> MNHLGKTEVFLNRFALRPLNPEELRPWRLEVVLDPPPGREEVYPLLAQVARRAGGVTVRMGDGLASWSPPEVLVLEGTLARMGQTYAYRLYPKGRRPLDPKDPGERSVLSALARRLLQERLRRLEGVWVEGLAVYRREHARGPGWRVLGGAVLDLWVSDSGAFLLEVDPAYRILCEMSLEAWLAQGHPLPKRVRNAYDRRTWELLRLGEEDPKELPLPGGLSLLDYH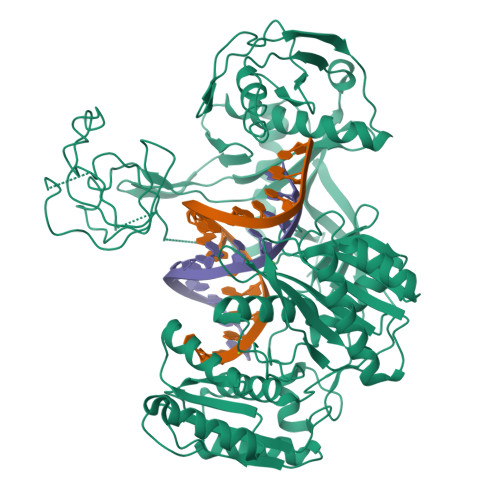ASKGRLQGREGGRVAWVADPKDPRKPIPHLTGLLVPVLTLEDLHEEEGSLALSLPWEERRRRTREIASWIGRRLGLGTPEAVRAQAYRLSIPKLMGRRAVSKPADALRVGFYRAQETALALLRLDGAQGWPEFLRRALLRAFGASGASLRLHTLHAHPSQGLAFREALRKAKEEGVQAVLVLTPPMAWEDRNRLKALLLREGLPSQILNVPLREEERHRWENALLGLLAKAGLQVVALSGAYPAELAVGFDAGGRESFRFGGAACAVGGDGGHLLWTLPEAQAGERIPQEVVWDLLEETLWAFRRKAGRLPSRVLLLRDGRVPQDEFALALEALAREGIAYDLVSVRKSGGGRVYPVQGRLADGLYVPLEDKTFLLLTVHRDFRGTPRPLKLVHEAGDTPLEALAHQIFHLTRLYPASGFAFPRLPAPLHLADRLVKEVGRLGIRHLKEVDREKLFFV Kinesins are a superfamily of microtubule (MT)-based molecular motors that play important roles in cellular functions such as mitosis, cell motility, and intracellular transport. The kinesin motor domain is the MT-binding engine that drives these activities, converting the chemical energy of ATP binding and hydrolysis into mechanical force. Recently, it has been demonstrated that a subset of kinesin superfamily members, including kinesin-2s, −3 s, −8 s, and −12 s, are sequestered by kinesin-binding protein (KBP; KIF1BP; KIAA1279), which inhibits MT track attachment by their motor domains and, thus, blocks their MT-related functions. Here we present cryo-electron microscopy (cryo-EM) structures of KBP alone and of KBP bound to the motor domain of the human mitotic kinesin KIF15 (a 110 kDa complex).

To elucidate the mechanism of kinesin inhibition by KBP, we determined the structure of KBP in complex with the human KIF15 (kinesin-12) motor domain (KIF15_MD, 1–375). The overall resolution of this KBP–KIF15_MD6S complex was 6.9 Å, with KBP and KIF15_MD6S determined to similar local resolutions. We built a model of the complex via flexible fitting using our KBP model and the KIF15_MD crystal structure. The complex is arranged such that KIF15_MD6S sits in the concave face of the KBP α-solenoid, analogous to a baseball enclosed in a baseball glove. When the structure of KBP-alone is superimposed onto KBP in the KBP–KIF15_MD6S complex, it is clear that KBP undergoes a conformational change in the presence of its kinesin motor domain-binding partner, with the largest differences resulting from an unfurling motion of its N-terminal subdomain. The structure of the KBP–KIF15_MD6S complex revealed that KBP binds the kinesin motor domain via the tubulin-binding subdomain. While the P-loop and Switch 1/2 subdomains of the KIF15_MD crystal structure and associated Mg2+-ADP generally fitted well into density of the KBP–KIF15_MD6S complex, a large portion of the tubulin-binding subdomain did not. In particular, there is a striking lack of density in the expected position for helix α4. Instead, there was a strong density of length and width consistent with helix α4 displaced by ~15 Å into the concave face of KBP, which we modelled as such. This displacement of helix α4, which lies close to the TPR-repeat region of the N-terminal subdomain of KBP, is accompanied by additional rearrangements of the flanking L11 and L12 in KIF15_MD6S (labelled KL11 and KL12).

> MANVPWAEVCEKFQAALALSRVELHKNPEKEPYKSKYSARALLEEVKALLGPAPEDEDERPEAEDGPGAGDHALGLPAEVVEPEGPVAQRAVRLAVIEFHLGVNHIDTEELSAGEEHLVKCLRLLRRYRLSHDCISLCIQAQNNLGILWSEREEIETAQAYLESSEALYNQYMKEVGSPPLDPTERFLPEEEKLTEQERSKRFEKVYTHNLYYLAQVYQHLEMFEKAAHYCHSTLKRQLEHNAYHPIEWAINAATLSQFYINKLCFMEARHCLSAANVIFGQTGKISATEDTPEAEGEVPELYHQRKGEIARCWIKYCLTLMQNAQLSMQDNIGELDLDKQSELRALRKKELDEEESIRKKAVQFGTGELCDAISAVEEKVSYLRPLDFEEARELFLLGQHYVFEAKEFFQIDGYVTDHIEVVQDHSALFKVLAFFETDMERRCKMHKRRIAMLEPLTVDLNPQYYLLVNRQIQFEIAHAYYDMMDLKVAIADRLRDPDSHIVKKINNLNKSALKYYQLFLDSLRDPNKVFPEHIGEDVLRPAMLAKFRVARLYGKIITADPKKELENLATSLEHYKFIVDYCEKHPEAAQEIEVELELSKEMVSLLPTKMERFRTKMALT;> MAPGSKTELRSVTNGQSNQPSNEGDAIKVFVRIRPPAERSGSADGEQNLSLSVLSSTSLRLHSNPEPKTFTFDHVADVDTTQESVFATVAKSIVESCMSGYNGTIFAYGQTGSGKTFTMMGPSESDNFSHNLRGVIPRSFEYLFSLIDREKEKAGAGKSFLSKCSFIEIYNEQIYDLLDSASAGLYLREHIKKGVFVVGAVEQVVTSAAEAYQVLSGGWRNRRVASTSMNRESSRSHAVFTITIESMEKCNEIVNIRTSLLNLVDLAGSERQKDTHAEGMRLKEAGNINRSLSTLGQVITALVDVGNGKQRHVSYRDSKLTFLLRDSLGGNAKTAIIANVHPGSRSFGETLSTLNFAQRAKLIKNKAVVNEDTQCLEHHHHHH> GHHHHHHML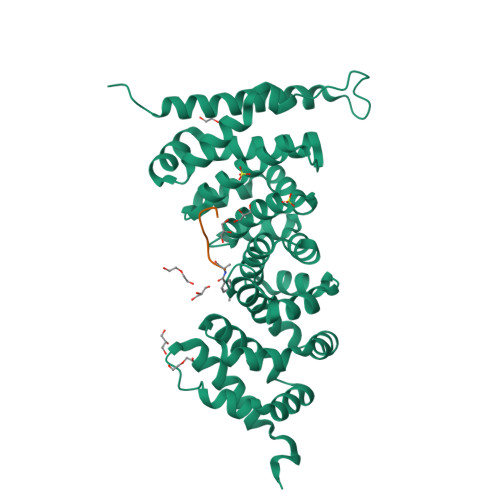HLLEQIRAYCETCWEWQEAHEPGMDQDKNPMPAPVEHQICPAVCVLMKLSFDEEHRHAMNELGGLQAIAELLQVDCEMYGLTNDHYSITLRRYAGMALTNLTFGDVANKATLCSMKGCMRALVAQLKSESEDLQQVIASVLRNLSWRADVNSKKTLREVGSVKALMECALEVKKESTLKSVLSALWNLSAHCTENKADICAVDGALAFLVGTLTYRSQTNTLAIIESGGGILRNVSSLIATNEDHRQILRENNCLQTLLQHLKSHSLTIVSNACGTLWNLSARNPKDQEALWDMGAVSMLKNLIHSKHKMIAMGSAAALRNLMANRPAKYKDANIMSPGSSLPS>MLYKLLNVLWLVAVSNAIPGTPVIDWADRNYALVEINYEATAYENLIKPKEQVDVQVSWNVWNGDIGDIAYVLFDEQQVWKGDAESKRATIKVLVSGQFNMRVKLCNEDGCSVSDPVLVKVADTDGGHLAPLEYTWLENNKPGRREDKIVAAYFVEWGVYGRNFPVDKVPLPNLSHLLYGFIPICGGDGINDALKTISGSFESLQRSCKGREDFKVAIHDPWAAVQKPQKSVSAWNEPYKGNFGQLMAAKLANPHLKILPSIGGWTLSDPFYFMHDVEKRNVFVDSVKEFLQVWKFFDGVDVDWEFPGGKGANPSLGDAERDAKTYILLLEELRAMLDDLEAQTGRVYEL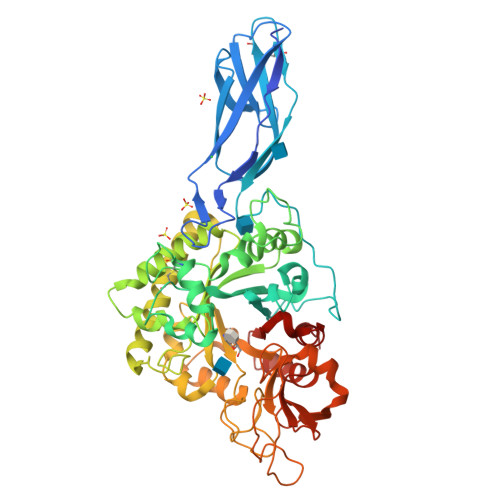TSAISAGYDKIAVVNYAEAQKSLGKIFLMSYDFKGAWSNTDLGYQTTVYAPSWNSEELYTTHYAVDALLKQGVDPNKIIVGVAMYGRGWTGVTNYTNDNYFSGTGNGPVSGTWEDGVVDYRQIQKDLNNYVYTFDSAAQASYVFDKSKGDLISFDSVDSVLGKVKYVDRNKLGGLFAWEIDADNGDLLNAINAQF[2x]> GRRTVPRGTLRKIIKKHKPHLRLAANTDLLVHLSFLLFLHRLAEEARTNAFENKSKII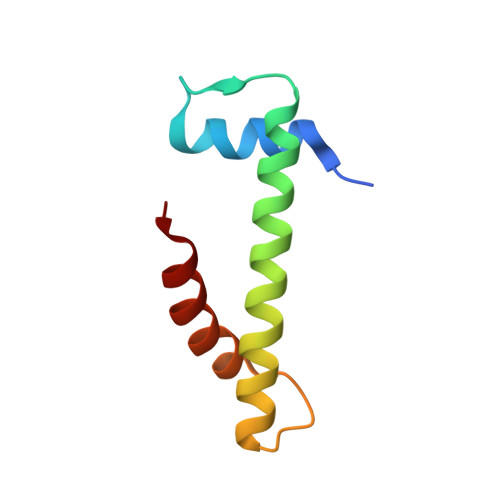KPEHTIAAAKVILKKSRG>[2x]VKPLQVEPPEPVVAVALGASRQLTCRLACADRGASVQWRGL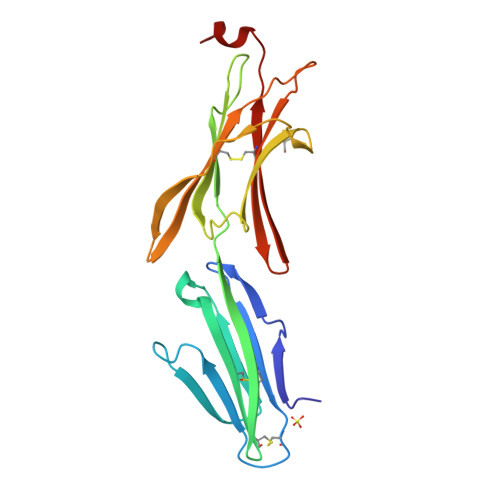DTSLGAVQSDTGRSVLTVRNASLSAAGTRVCVGSCGGRTFQHTVQLLVYAFPNQLTVSPAALVPGDPEVACTAHKVTPVDPNALSFSLLVGGQELEGAQALGPEVQQEPIGGDVLFRVTERWRLPPLGTPVPPALYCQATMRLPGLELSHRQAIPVLGGENLYFQ>[4x]SNAMFAPQGLAQFIKVNVTLENGEPVFIYTDANGQVCQGAITVTQAGTITYLLNDQTLKGLKFVGVGFVTPFDGIIDAVTISSDGMLVQLVD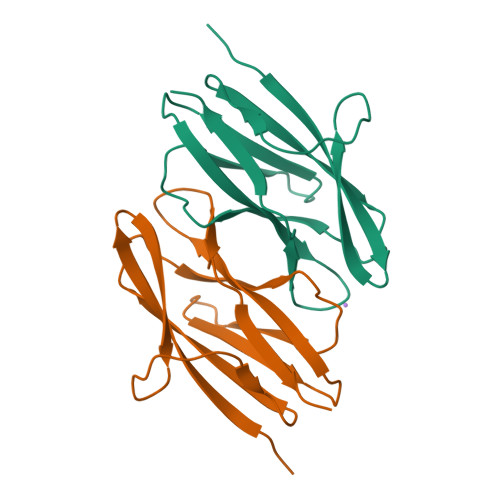LDKTPGTTKFQFVLSNTANTLLVLSPDPQIINRPQN>MTHELISLPYAVDALAPVISKETVEFHHGKHLKTYVDNLNKLIIGTEFENADLNTIVQKSEGGIFNNAGQTLNHNLYFTQFRPGKGGAPKGKLGEAIDKQFGSFEKFKEEFNTAGTTLFG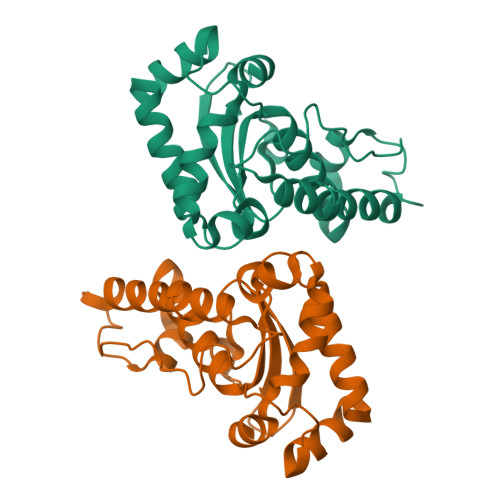SGWVWLASDANGKLSIEKEPNAGNPVRKGLNPLLGFDVWEHAYYLTYQNRRADHLKDLWSIVDWDIVESRY[4x]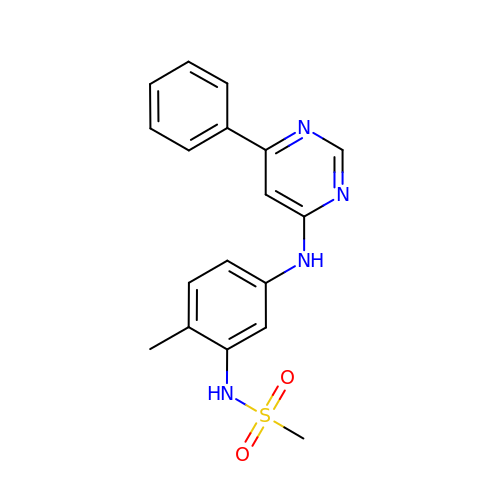N-{2-methyl-5-[(6-phenylpyrimidin-4-yl)amino]phenyl}methanesulfonamide | C18 H18 N4 O2 S | CXQRKICWSCAUGW-UHFFFAOYSA-N> AAQTNAPWGLARISSTSPGTSTYYYDESAGQGSCVYVIDTGIEASHPEFEGRAQMVKTYYYSSRDGNGHGTHCAGTVGSRTYGVVKKTQLFGVKVLDDNGSGQYSTIIAGMDFVASDKNNRNCPKGVVASLSLGGGYSSSVNSAAARLQSSGVMVAVAAGNNNADARNYSPASEPSVCTVGASDRYDRRSSFSNYGSVLDIFGPGTSILSTWIGGSTRSISGTSMATPHVAGLAAYLMTLGKTTAASACRYIADTANKGDLSNIPFGTVNLLAY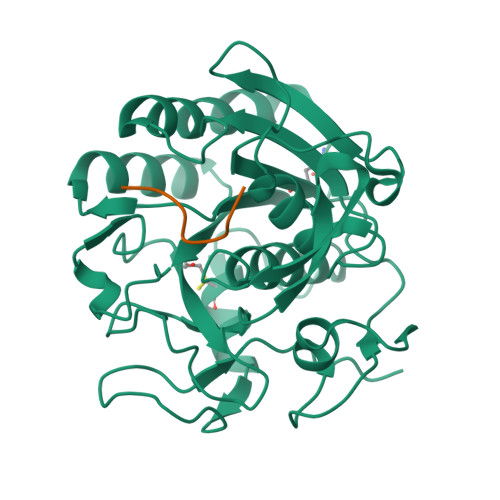NNYQA;> XPAPFAAAAX> AGAGAGAGAGMDVPLMELSGRAPVVRLHDIEADMAAATDAIRSQLTGWGFMAAEVPGIGERVEAMMNEFAAACRATGPSLSDYAYDVVPQLAVGGTHGFFPYNSEIPRLANGVPDPKEFIHVSGAMIGDQPPGAGDVLRAFPAFGTRAAEVFDIAFRLISLFGEVVRGMMPPGTPELDLSHDATNLRVIHYRDVGDREVL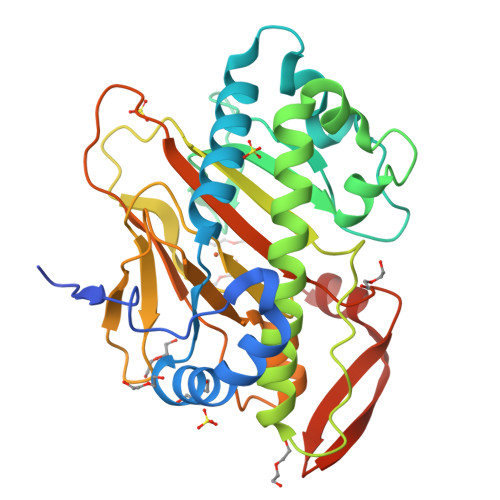AHEHSGIQMLGLQLPPSDQGLQYVLHDGTWVEPVIAGTDVVLCNIGRMLTSASDGRFRPSTHRVHTKPMPAGYERLSSVLFAYPQHKARQWKMVDGELMSLNATWGDFIDSRFQGLGKQS>GPGMKFKIDYELPLTSVAGKIRIKQRSTFNDYGLPVAPTKININVKHYVEWQIGYDMVAGKNDGNFIGANGKDKKLYELSDIIFQFFKHNIILKENLFGIKNFLENNEELIEDKMKINRTNFTQKQVAGINFLESYVSYPLLVYQFNNNEF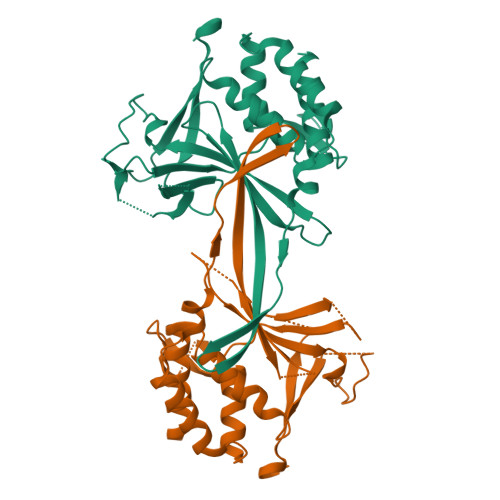LSEIIIKEKQRAIGVQGMLYFCFPVHLLKNINGERNFLNRSIESKEKGYLEISRNNINIFLEMLKIFGILSNNHRYNVLQIIEFILNSK[2x]> MVDSRNADTEQENENLSKFCIDMTAMAREGKIDPVIGREEEIRRVIRILSRRTKNNPVLIGEPGVGKTTIVEGLAQRIVNADVPDNLAACKLLSLDVGALVAGSKYRGEFEERMKGVLKEIQESKETIILFVDEIHLLMGAGSSGEGGMDAANLLKPMLARGQLHCIGATTLAEYRKYIEKDAAFERRFQQVLVKEPSITETISILRGLKEKYEVHHGVNIADAAIVAAANLAARYLTSRRLPDSAVDLIDEAAAAVRVARESQPEIIDSLERRLRQLKIEIHALSREKDEASKARLAQAKQDAQNVEEELRPLREKYERERQRGKAIQEAKMKLEALRVKAEDASRMGDHSRAADLQYYAIPEQEAIIKRLEAEKAAADAALNANGADVGGSMITDVVGPDQINEIVARWTGIPVTRLKTSEKEKLLHMEQALSKIVVGQKEAVQSVSNAIRLQRSGLSNPNQPPSFLFCGPSGTGKTLLTKALAEFLFDDPKSMIRFDMSEYQERHSLSRMIGAPPGYVGHDAGGQLTEALRRRPFSILLFDEVEKAAKEVLTVLLQLMDDGRITDGQGRVVDAKNCIVVMTSNLGAEYLSRANNGKDGKIDPTTRELVMNTLRNYFLPEFLNRISSIVIFNRLTRREIR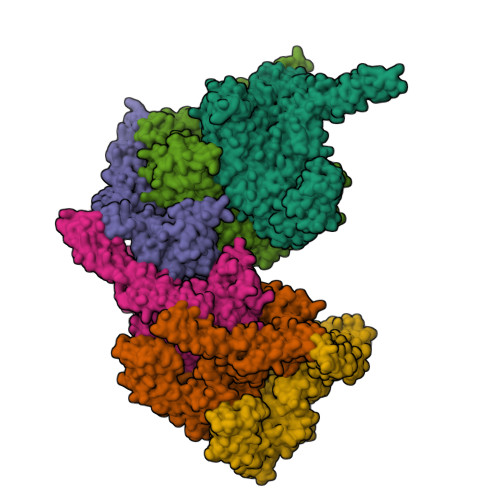KIVDLRIAEIQKRLTDNDRNVTIKVSDEAKDKLGAQGYSPVYGARPLQRLLEKEVLNRLAILILRGQIREGEVACVELVDGKVQVLPNHPDSEPEDVDVDMESDDAVDEVAPDSMDEDIYND>[2x]HMVSLTERRKAETRMEIARAAARLFVGQGLRATRAEDIARAAGVAPRTFYRYFATKEE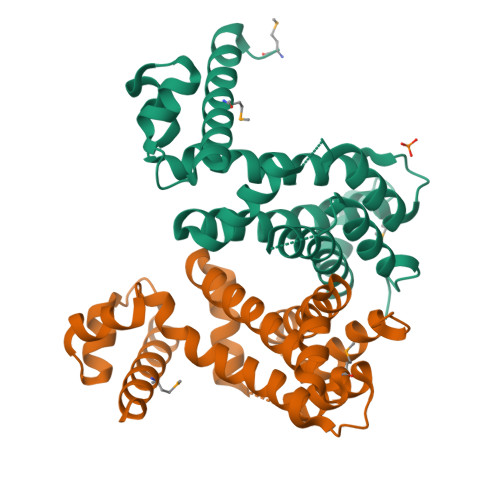AVAPLYALGAERWVRAVREAPAELSPPEALERAVRHTLTPGAGVSAPSWEWARTLIRLAESSPALRKVWAEVCHSTERGLVQALAARMSGGDDNVAVRLAASPRLHFAAAVAGASVRVAAEHWASSSPQGARSPLEQALLNLEVLRGFAWEAGPAEEG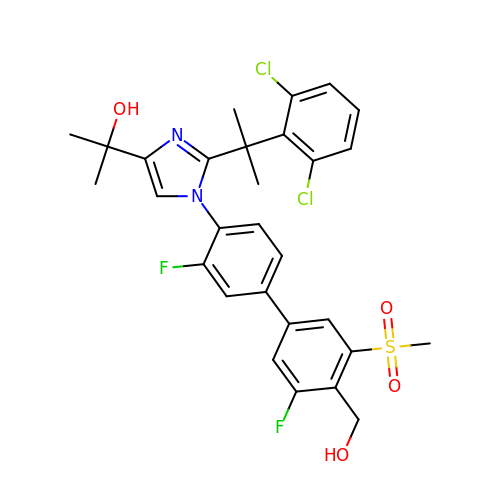2-[2-[2-[2,6-bis(chloranyl)phenyl]propan-2-yl]-1-[2-fluoranyl-4-[3-fluoranyl-4-(hydroxymethyl)-5-methylsulfonyl-phenyl]phenyl]imidazol-4-yl]propan-2-ol | C29 H28 Cl2 F2 N2 O4 S | HNAJDMYOTDNOBK-UHFFFAOYSA-N ZIP4 is the exclusive zinc transporter specifically expressed on the apical surface of intestinal epithelium and responsible for dietary zinc absorption. ZIP4 knockout in mouse is embryonic lethal, and loss-of-function mutations of ZIP4 lead to a lethal genetic disorder, Acrodermatitis Enteropathica (AE). Structurally, the LIV-1proteins share a similar topology: a transmembrane domain (TMD) with predicted eight transmembrane helices and a large and variable N-terminal extracellular domain (ECD). In this work, we present the first crystal structure of a mammalian ZIP4-ECD at a resolution of 2.8 Å, which reveals an unprecedented dimer centred at the signature PAL motif.

A ZIP4-ECD from Pteropus Alecto (black fruit bat, pZIP4-ECD) was found to have ideal behaviour in solution. pZIP4-ECD shares 68% identical residues with human ZIP4-ECD, and cell-based zinc uptake assay confirmed that the full-length pZIP4 is a functional zinc transporter. In one asymmetric unit, two pZIP4-ECD molecules form a homodimer. The structure of pZIP4-ECD shows that each protomer has two structurally independent subdomains. The structure of pZIP4-ECD is stabilized by four disulfide bonds (C59–C64, C67–C103, C153–C188 and C266–C305). Two pZIP4-ECD molecules form an elongated and wing-shaped dimer: the two PCDs pack together and form a central dimeric module, which is flanked by two HRDs forming the ends of the wing. Structure superimposition of the PCDs reveals that the HRD of molecule B (HRDB) rotates, from the position of the HRDA, ∼20° relative to the PCD dimer, suggestive of structural flexibility of the bridging region. Most interestingly, the absolutely conserved proline residue (P294) in the PAL motif, together with a highly conserved serine residue (S293), are located at the cross of the two α14s which are at the centre of the PCD dimer.

>[2x]SGQGALDRVALGGLLNTLAARVHCTSGPCGKCLSVDDLLALGRPEEPGHLARLSAAAALYLSDPEGTCEDIRAGRWASRADHLLALLEGPKALAPGLSRLLQRIQAQTTGQPSAGEACVDPPQLLREAGVAGAPGSPGPVLATLLEHVGRGSCFHTLPTPQYFVDFVFQQSHGNTPNISVAELAALMQRLGVGGVTETHSDHHHQEKRVNRQGPTPLTAPNSSSDTWDTVCLSARDVMAVYGLSEQTGVTPEAWAQLSPALLQQQLSGACSPQPSHPAQNQLSQAEK>GPRMAFTNYSSLNRAQLTFEYLHTNSTTHEFLFGALAELVDNARDADATRIDIYAERREDLRGGFMLCFLDDGAGMDPSDAASVIQFGKLAKRTPESTQIGQYGNGLKSGSMRIGKDFILFTKKEDTMTCLFLSRTFHEEEGIDEVIVPLPTWNARTREPVTDNVEKFAIETELIYKYSPFRTEEEVMTQFMKIPGDSGTLVIIFNLKLMDNGEPELDIISNPRDIQMAETSPEGTKPERRSFRAYAAVLYIDPRMRIFIHGHKVQTKRLSCCLYKPRMYKYTSSRFKTRAEQEVKKAEHVARIAEEKAREAESKARTLEVRLGGDLTRDSRVMLRQVQNRAITLRREADVKKRIKEAKQRALKEPKELNFVFGVNIEHRDLDGMFIYNCSRLIKMYEKVGPQLEGGMACGGVVGVVDVPYLVLEPTHNKQDFADAKEYRHLLRAMGEHLAQYWKDIAIAQRGIIKFWDEFGYLSANWNQPPSSELRYKRRRAMEIPTTIQCDLCLKWRTLPFQLSSVEKDYPDTWVCSMNPDPE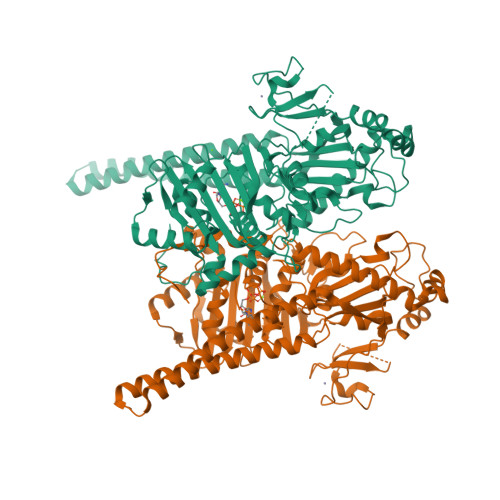QDRCEASEQKQKVPLGTFRKDMKTQEEKQKQLTEKIRQQQEKLEALQKTTPIRSQADLKKLPLEVTTRPST[2x]> EATAGTVTVNAITSDDTIDGIELGQTISISGKAVGGDISVGDVVKMTINNTEYSTTVKAGGIWMIAGVLGSDLAADSEFDVVVTSSDAAGNKVQSIGTSTHSVDLSAEANFSLAEGQQHVLTNLPEGFGFPDGTTEVVTNFGGTITLGDDGEYRYDAPVRDHGDAVSDKDSVTVTLEDGRTFTVNLDIQDSAPVAVDDQDSIVVQHEEFEVSEIAASWVSYTHGESVTTFDGTSDLGGVDNDSAKDQIRWGNPAESKQSGYGFIDNDSNLEGRFDLNQDISVGT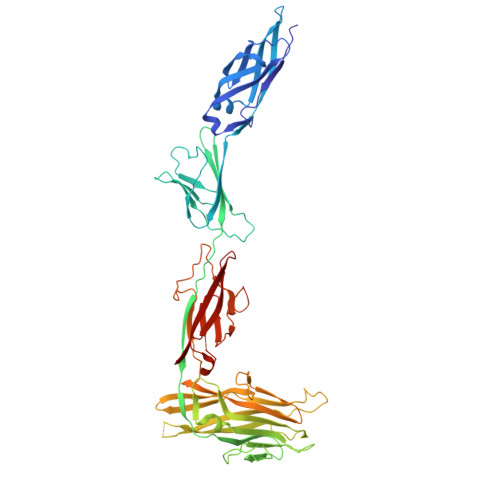FTHYNYPVYSGGAITSAEMSVEFSVLDHLGVSTPVTLTVNFDHNETPNTNDVNASRDIVTVQNTHVTFERDGDIYTVQIVGFREVGNPDGEVVTSIYTNENAATSYELVVRVVEGDGYSLPSTEGNIFDDNGLGADSLGADGSVTVVGVAVGAIVSSNESVGHSIEGQYGNLVLNSDGSYVYDVTASVSDIPAGATESFAYLIQDQDGSTSSANLSINVGTN>MNNFGNEEFDCHFLDEGFTAKDILDQKINEVSSSDDKDAFYVADLGDILKKHLRWLKALPRVTPFYAVKCNDSKAIVKTLAATGTGFDCASKTEIQLVQSLGVPPERIIYANPCKQVSQIKYAANNGVQMMTFDSEVELMKVARAHPKAKLVLRIATDDSKAVCRLSVKFGATLRTSRLLLERAKELNIDVVGVSFHVGSGCTDPETFVQAISDARCVFDMGAEVGFSMYLLDIGGGFPGSEDVKLKFEEITGVINPALDKYFPSDS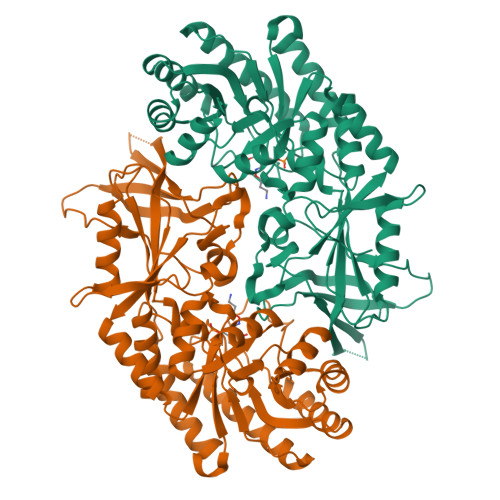GVRIIAEPGRYYVASAFTLAVNIIAKKIVLKEQTGSDDEDESSEQTFMYYVNDGVYGSFNCILYDHAHVKPLLQKRPKPDEKYYSSSIWGPTCDGLDRIVERCDLPEMHVGDWMLFENMGAYTVAAASTFNGFQRPTIYYVMSGPAWQLMQQFQNPD[2x]>[2x]SNAMKTVTVRDLVVGEGAPKIIVSLMGKTITDVKSEALAYREADFDILEWRVDHFANVTTAESVLEAAGAIREIIT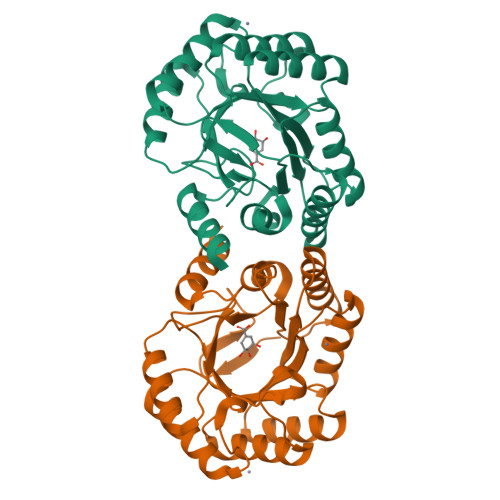DKPLLFTFRSAKEGGEQALTTGQYIDLNRAAVDSGLVDMIDLELFTGDDEVKATVGYAHQHNVAVIMSNHDFHKTPAAEEIVQRLRKMQELGADIPKIAVMPQTKADVLTLLTATVEMQERYADRPIITMSMSKTGVISRLAGEVFGSAATFGAVKKASAPGQISVADLRTVLTILHQA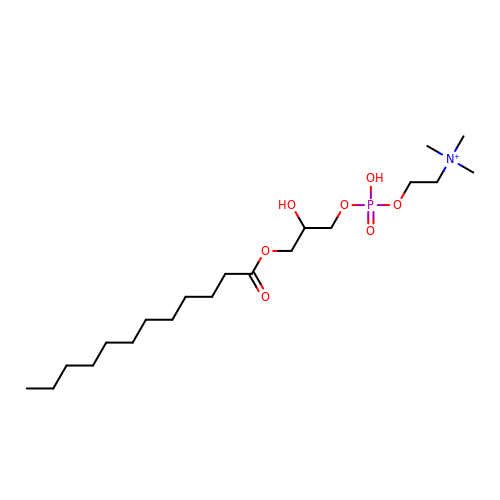[2-((1-OXODODECANOXY-(2-HYDROXY-3-PROPANYL))-PHOSPHONATE-OXY)-ETHYL]-TRIMETHYLAMMONIUM | C20 H43 N O7 P | BWKILASWCLJPBO-UHFFFAOYSA-O> GPISSKPVIVTGLQDTTVSSDSVAKFAVKATGEPRPTAIWTKDGKAITQGGKYKLSEDKGGFFLEIHKTDTS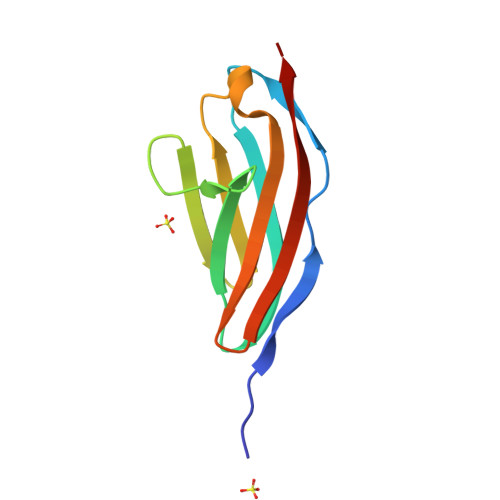DSGLYTCTVKNSAGSVSSSCKLTIKAI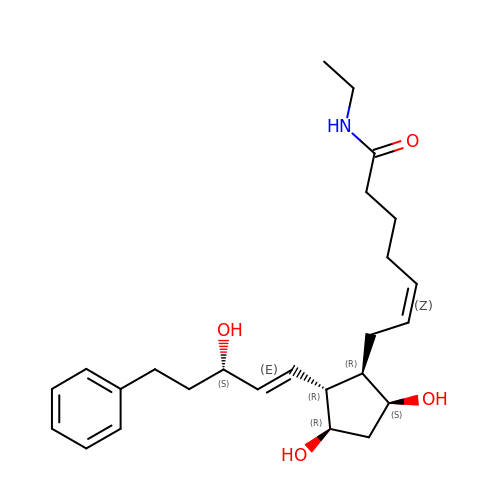(5Z)-7-{(1R,2R,3R,5S)-3,5-DIHYDROXY-2-[(1E,3S)-3-HYDROXY-5-PHENYLPENT-1-ENYL]CYCLOPENTYL}-N-ETHYLHEPT-5-ENAMIDE | C25 H37 N O4 | AQOKCDNYWBIDND-FTOWTWDKSA-N>[6x]HPSSPPVVDTVHGKVLGKFVSLEGFAQPVAIFLGIPFAKPPLGPLRFTPPQPAEPWSFVKNATSYPPMCTQDPKAGQLLSELFTNRKENIPLKLSEDCLYLNIYTPADLTKKNRLPVMVWIHGGGLMVGAASTYDGLALAAHENVVVVTIQYRLGIWGFFSTGDEHSRGNWGHLDQVAALRWVQDNIASFGGNPGSVTIFGESAGGESVSVLVLSPLAKNLFHRAISESGVALTSVLVKKGDVKPLAEQIAITAGCKTTTSAVMVHCLRQKTEEELLETTLKMKFLSLDLQGDPRESQPLLGTVIDGMLLLKTPEELQAERNFHTVPYMVGINKQEFGWLIP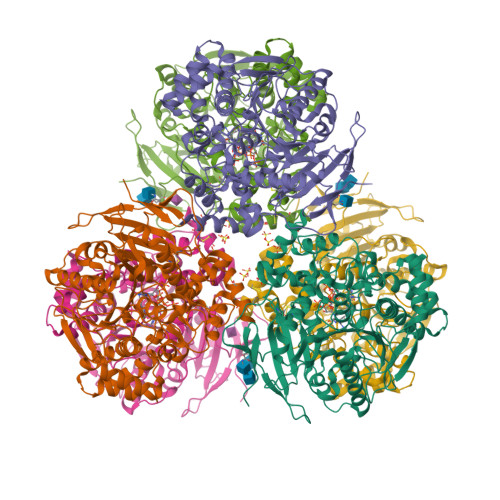MLMSYPLSEGQLDQKTAMSLLWKSYPLVCIAKELIPEATEKYLGGTDDTVKKKDLFLDLIADVMFGVPSVIVARNHRDAGAPTYMYEFQYRPSFSSDMKPKTVIGDHGDELFSVFGAPFLKEGASEEEIRLSKMVMKFWANFARNGNPNGEGLPHWPEYNQKEGYLQIGANTQAAQKLKDKEVAFWTNLFAKKAVEKPPQ>[2x]MGAEEELKVEVKELTPPVISLALPSQGLKVVRNTDYTFTPDIQHSDVEGFKIEWVREGKIVSTENTYTFNEKELGVYTVTINASN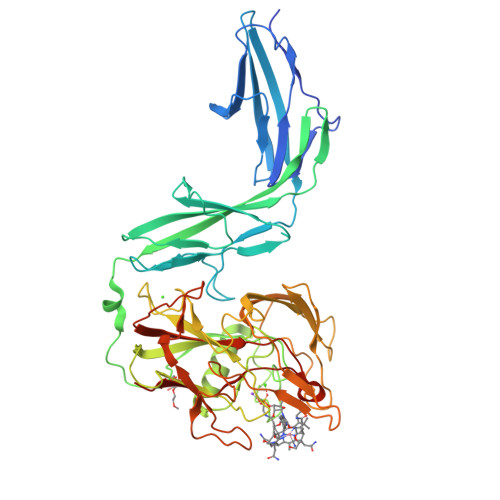IDGTTTKDVSVEVVETMPYVVKFPTPSYLQTSTDRYTFADRPVFLRPLLEYFDNPRFEWSVDGQVMEGEVERMFKFTPSAPGEYTVSCTVSEDTPTEKISRNIDKGKTAVTATVKVVCVDKKEQDGFRASGSSKLWNKVYEYTPAPGQFINETSTIGGMTGNETSPEAAVAWATQRLKDKLHVSLGSFGGYIIVGFDHSIPNSGNQYDFCVQGNAFDGSSEPGIVWVMQDINGNGLPDDEWYELKGSEAGKEETIQNFEVTYYRPEGKKMDVQWISSDGRNGWVDYLSAYHTQDYYYPAWISENSYTLTGTCLAARNTQDSQTGYWDNQSYDWGYVDNFGNDQIEGGSTVDGSGQRNGFKISNAIHADGTEANLQYIDFIKIQCGVLAKSGWLGEVSTEVFSFEDLTKLEHHHHHH> MILDTDYITEDGKPVIRIFKKENGEFKIDYDRNFEPYIYALLKDDSAIEDVKKITAERHGTTVRVVRAEKVKKKFLGRPIEVWKLYFTHPQDQPAIRDKIKEHPAVVDIYEYDIPFAKRYLIDKGLIPMEGDEELKMLAFAIATLYHEGEEFAEGPILMISYADEEGARVITWKNIDLPYVDVVSTEKEMIKRFLKVVKEKDPDVLITYNGDNFDFAYLKKRSEKLGVKFILGREGSEPKIQRMGDRFAVEVKGRIHFDLYPVIRRTINLPTYTLEAVYEAIFGQPKEKVYAEEIAQAWETGEGLERVARYSMEDAKVTYELGKEFFPMEAQLSRLVGQSLWDVSRSSTGNLVEWFLLRKAYERNELAPNKPDERELARRRESYAGGYVKEPERGLWENIVYLDFRSLYPSIIITHNVSPDTLNREGCEEYDVAPQVGHKFCKDFPGFIPSLLGDLLEERQKVKKKMKATIDPIEKKLLDYRQRLIKILANSFYGYYGYAKARWYCKECAESVTAWGRQYIETTIREIEEKFGFKVLYADTDGFFATIPGADAETVKKKAKEFLDYINAKLPGLLELEYEGFYKRGFFVTKKKYAVIDEEDKITTRGLEIVRRDWSEIAKETQARVLEAILKHGDVEEAVRIVKEVTEKLSKYEVPPEKLVIYEQITRDLKDYKATGPHVAVAKRLAARGIKIRPGTVISYIVLKGSGRIGDRAIPFDEFDPAKHKYDAEYYIENQVLPAVERILRAFGYRKEDLRYQKTRQVGLGAWLKPKT

Archaeal DNA polymerases from the B-family (polB) have found essential applications in biotechnology. Variants of the archaeal polymerase from Thermococcus gorgonarius, TgoT, that can either generate HNA from DNA (TgoT_6G12) or DNA from HNA (TgoT_RT521) have been previously identified. In this study, six X-ray structures of DNA and HNA polymerases are reported: (i) three apo- structures of TgoT, TgoT_6G12, and TgoT_RT521-; (ii) two DNA-bound structures of TgoT_6G12 in binary and ternary complexes; and (iii) one DNA-bound structure of TgoT_6G12, which has incorporated two HNA nucleotides. Consistent with all other DNAPs from B-family, TgoT and its variants fold into five distinct structural subdomains.

In particular, the compartmentalized self-tagging (CST) strategy enabled the discovery of polymerases capable of processive HNA synthesis. This approach was performed on libraries of mutants of a variant of the replicative B-family DNAP, which was isolated from the archaeal hyperthermophilic Thermococcus gorgonarius (Tgo). To better understand how the mutations added on TgoT variants impact the structure of the polymerase, the X-ray structures of the apo form of TgoT, replicative polymerase TgoT_6G12, and reverse transcriptase TgoT_RT521 were solved by crystallography. Crystals were obtained for the three polymerases and diffracted at 2.4, 3.1, and 2.35 Å, respectively. The helices α19 and α20 are part of these regions. Hence, overall, the crystal structure of the wild-type TgoT appears more stable than the two variants studied here. For instance, compared to their initial position in the Tgo DNAP structure, helices α19 and α20 of the thumb β subdomain of TgoT shift by almost 5.5 and 6 Å, respectively. Nevertheless, both structures are in the known and expected “open” conformation. The presence of this antechamber, which is reminiscent of a storage pocket, was actually observed in two other structures, namely the apo-structure of TgoT and the binary structure of TgoT_6G12, all grown in an excess of ddNTP.> MEPHSLRYNLMVLSQDESVQSGFLAEGHLDGQPFLRYDRQKRRAKPQGQWAEDVLGAETWDTETEDLTENGQDLRRTLTHIKDQKGGLHSLQEIRVCEIHEDSSTRGSRHFYYNGELFLSQNLETQESTVPQ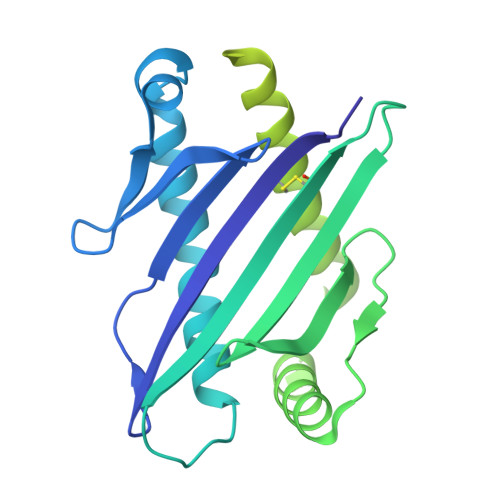SSRAQTLAMNVTNFWKEDAMKTKTHYRAMQADCLQKLQRYLKSGVAIRRTVPPMVNVTCSEVSEGNITVTCRASSFYPRNITLTWRQDGVSLSHNTQQWGDVLPDGNGTYQTWVATRIRQGEEQRFTCYMEHSGNHGTHPVPSGKVLVLQSQRTDFPYVSAAMPCFVIIIILCVPCCKKKTSAAEGP N-methyl-4,5-dihydrobenzo[g]benzothiophene-2-carboxamide 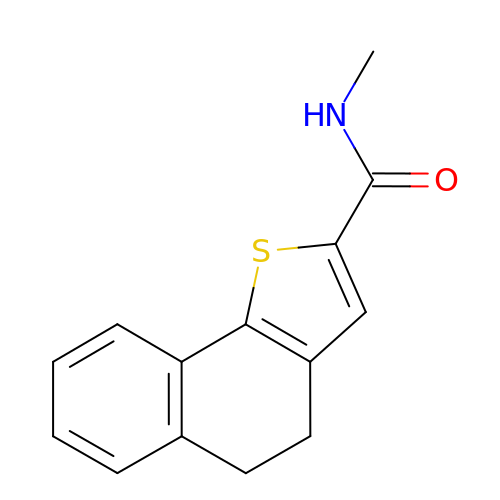| C14 H13 N O S | ADOUOUVBTDMDIV-UHFFFAOYSA-N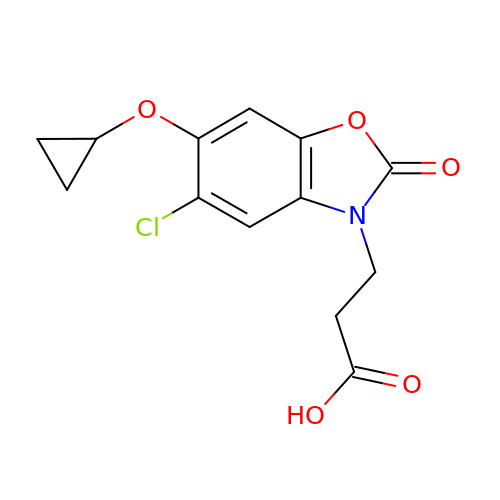3-(5-chloro-6-cyclopropoxy-2-oxo-2,3-dihydro-1,3-benzoxazol-3-yl)propanoic acid | C13 H12 Cl N O5 | AYXQPTCYJAJHBG-UHFFFAOYSA-N>CGCGAATTCGCG[2x]

The rational design of small molecules that target specific DNA sequences is a promising strategy to modulate gene expression. This report focuses on a diamidinobenzimidazole compound, whose selective binding to the minor groove of AT DNA sequences holds broad significance in the molecular recognition of AT-rich human promoter sequences. The specialized method of X-ray crystallography was utilized to investigate how the sequence-dependent recognition properties in general, A-tract, and alternating AT sequences affect the binding of diamidinobenzimidazole in the DNA minor groove. A strong and direct hydrogen bond between the N-H of the benzimidazole and an H-bond acceptor atom in the minor groove is essential for DNA recognition in all sequences described. In addition, the diamidine compound specifically utilizes an interfacial water molecule for its DNA binding.

The AATT-DB1476 complex structure reveals a unique 1:1 binding mode with two orientations of DB1476 observed in the minor groove. The electron density map of AATT-DB1476-I and AATT-DB1476-II does not show an unequivocal orientation assignment. Thus, we presented a structure with two possible ligand orientations. The significant difference between AATT-DB1476-I and AATT-DB1476-II is the flip of the amidine ends to an opposite orientation. AATT-DB1476-I and AATT-DB1476-II show identical interactions with the DNA bases at the minor groove. The BI-N-H in both complexes forms a strong direct H-bond in a bifurcated manner with the O2s of T7 and T19, respectively. In addition to the strong BI-N-H hydrogen bonds, one of the amidines in each complex, A-N6 in AATT-DB1476-I and C-N4 in AATT-DN1476-II, forms a strong direct hydrogen bond with O2 of C9. Similarly, in AATT-DB1476-II, the A-N6 forms a hydrogen bond with the O2 of T20 (−NH•••O – H•••O=T) via an interfacial water molecule. Based on the 1.63 Å resolution X-ray crystal structure of the AATT-DB1476-II, we also investigated the MD simulation of DB1476 with the 180° flip orientation. The MD simulation suggests that the two DB1476 orientations yield similar H-bonding interactions and hydration interactions, as observed in the X-ray structures.> MSRPRLNRLLVLEEAVRVADGAGGHRLDWQAK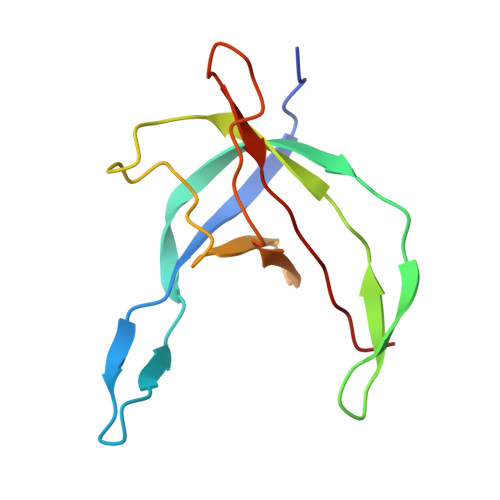GEVWAEVTAGSGSERAGEFVTLASVPFTIVVRAAPVGAARRPRPEQRFREGARIFRILAVAERDREGHYLSCFAREEVVA> MERKISRIHLVSEPSITHFLQVSWEKTLESGFVITLTDGHSAWTGTVSESEISQEADDMAMEKGKYVGELRKALLSGAGPADVYTFNFSKESAYFFFEKNLKDVSFRLGSFNLEKVENPAEVIRELIAYALDTIAENQAKNEHLQKENERLLRDWNDVQGRFEKAVSAKEALETDLYKRFILVLNEKKTKIRSLHNKLLNAAQEREKDIKQE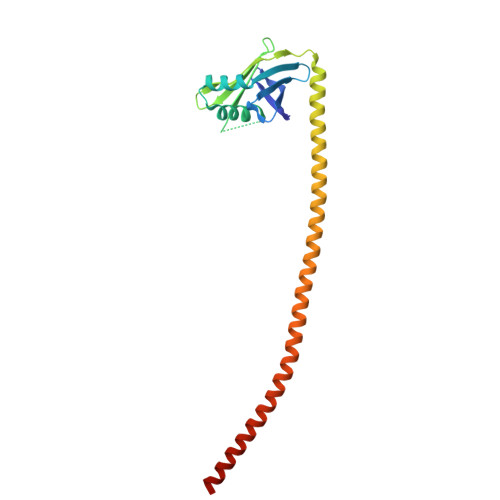G>[14x]MHRTYSLRNQRAPTAAELQAPPPPPSSTKSKFFGKASIASSFRKNAAGNFGPELARKLSQLVKTEKGVLRAMEVVASERREAAKQLSLWGADNDDDVSDVTDKLGVLIYELGELQDQFIDKYDQYRVTLKSIRNIEASVQPSRDRKEKITDEIAHLKYKDPQSTKIPVLEQELVRAEAESLVAEAQLSNITREKLKAAYSYMFDSLRELSEKFALIAGYGKALLELLDDSPVTPGEARPAYDGYEASRQIIMDAESALESWTLDMAAVKPTLSFHQTVDDVYEDEDGEEEEEPEIQNGDIPGQVVEEEEVEWTTEVPVDDEAHEADHHVSQNGHTSGSENI

The yeast eisosome, composed of the BAR-domain proteins Pil1 and Lsp1 (hereafter, Pil1/Lsp1), scaffolds a membrane compartment that senses and responds to mechanical stress by flattening and releasing sequestered factors. MCC–eisosomes are relatively stable, and have been implicated in sensing and responding to plasma membrane stress: various stimuli, including hypo-osmotic shock, heat shock and mechanical pressure, cause eisosomes to flatten and release sequestered proteins to affect signalling or transport functions. Here we isolated near-native eisosomes as helical tubules made up of a lattice of Pil1/Lsp1 bound to plasma membrane lipids, and solved their structures by helical reconstruction.

We isolated MCC–eisosomes from S. cerevisiae using a gentle purification procedure, preserving a lattice of untagged Pil1/Lsp1 structural proteins bound to a presumably intact plasma membrane bilayer in a near-native state, observable as a two-layer density in the protein tubule. Although MCC–eisosomes have been shown to have a furrow-like half-pipe structure in vivo, our isolated eisosome tubules seem to be closed, continuous helices of Pil1/Lsp1 proteins. Using a symmetry expansion and density subtraction strategy, we could refine our structures to a resolution of around 3.2 Å, which allowed us to build models of the paralogues Pil1 and Lsp1. Two novel structured regions of the protein were visible in our maps: (1) a folded N terminus (Nt) that forms lattice contact sites with the Nt of a neighbouring dimer, followed by (2) an Nt amphipathic helix (AH; residues 39–48) buried within the lipid density of the cytoplasmic leaflet of the bilayer that runs parallel to the BAR-domain helices of each Pil1/Lsp1 monomer.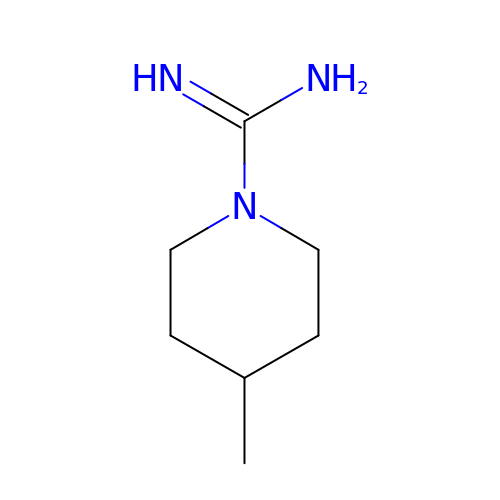4-methylpiperidine-1-carboximidamide | C7 H15 N3 | NIWNTTFADJMCIT-UHFFFAOYSA-N(3R,4R,5S)-4-acetamido-3-pentan-3-yloxy-5-(4-phenyl-1,2,3-triazol-1-yl)cyclohexene-1-carboxylic acid | C22 H28 N4 O4 | 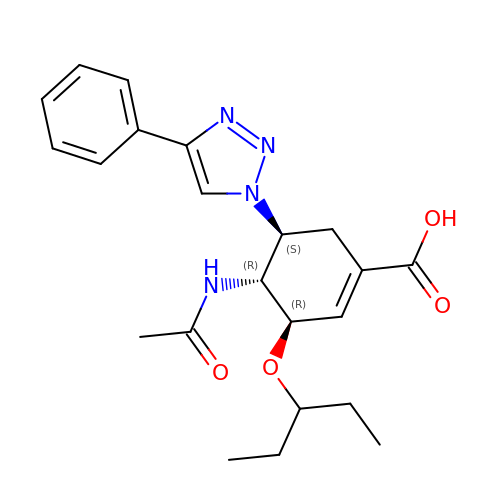GPEBJEGIHZQYIK-PWRODBHTSA-N>[3x]NIHKAQLNKNEERFKQLEGACYSGKLIWKVTDYRVKKREAVEGHTVSVFSQPFYTSRCGYRLCARAYLNGDGSGKGTHLS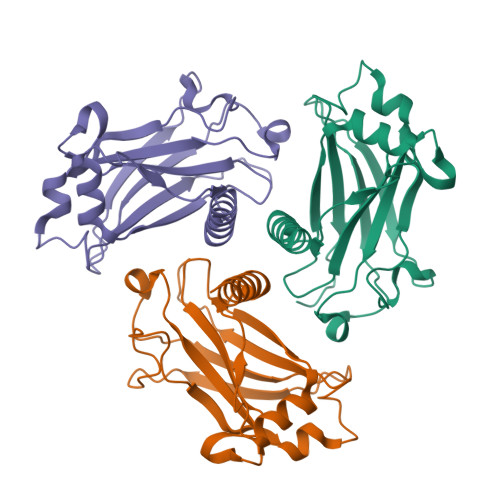LYFVVMRGEFDSLLQWPFRQRVTLMLLDQSGKKNHIVETFKADPNSSSFKRPDGEMNIASGCPRFVSHSTLENSKNTYIKDDTLFLKVAVDLTDLEDL> LAAAMLNLENKTYVIMGIANKRSIAFGVAKVLDQLGAKLVFTYRKERSRKELEKLLEQLNQPEAHLYQIDVQSDEEVINGFEQIGKDVGNIDGVYHSIAFANMEDLRGRFSETSREGFLLAQDISSYSLTIVAHEAKKLMPEGGSIVATTYLGGEFAVQNYNVMGVAKASLEANVKYLALDLGPDNIRVNAISAGPIRTLSAKGVGGFNTILKEIEERAPLKRNVDQVEVGKTAAYLLSDLSSGVT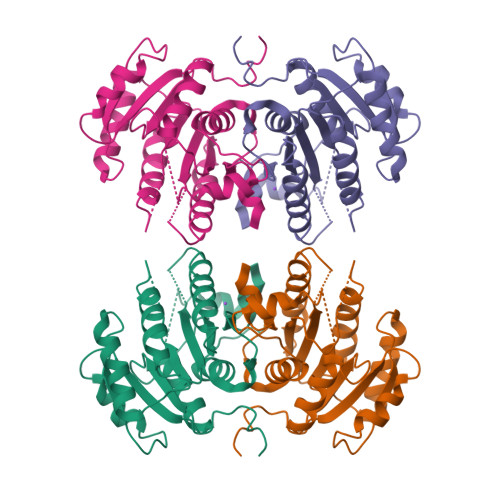GENIHVDSGFHAIK> MDVFAKHAVSLESPAVRHYEITPSDSTDLARRPRALRVQTGGTLVLRDETGITVTYTVFAGEILPVRPVRVLA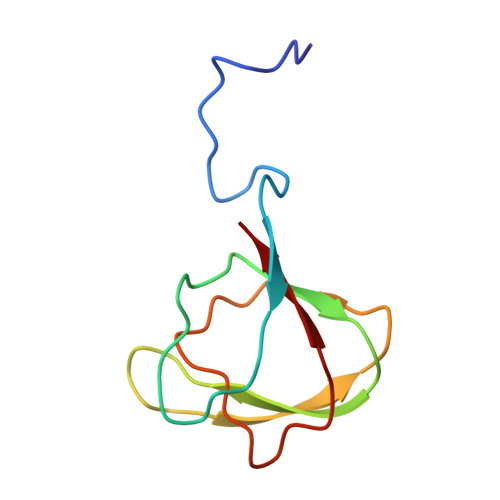TGTTATAVGWE>MLESKLKAPVFTATTQGDHYGEFVLEPLERGFGVTLGNPLRRILLSSIPGTAVTSVYIEDVLHEFSTIPGVKEDVVEIILNLKELVVRFLDPKMASTTLILRAEGPKEVRAGDFTPSADVEIMNPDLHIATLEEGGKLYMEVRVDRGVGYVPAERHGIKDRINAIPVDAIFSPVRRVAFQVEDTRLGQRTDLDKLTLRIWTDGSVTPLEALNQAVAILKEHLNYFANPEASLLPTPEVSKGEKRESAEEDLDLPLEELGLSTRVLHSLKEEGIESVRALLALNLKDLRNIPGIGERSLEEIRQALAKKGFTLKE[4x];>MEIKRFGRIREVIPLPPLTEIQVESYKKALQADVPPEKRENVGIQAAFKETFPIEEGDKGKGGLVLDFLEYRIGDPPFSQDECREKDLTYQAPLYARLQLIHKDTGLIKEDEVFLGHLPLMTEDGSFIINGADRVIVSQIHRSPGVYFTPDPARPGRYIASIIPLPKRGPWIDLEVEASGVVTMKVNKRKFPLVLLLRVLGYDQETLVRELSAYGDLVQGLLDEAVLAMRPEEAMVRLFTLLRPGDPPKKDKALAYLFGLLADPKRYDLGEAGRYKAEEKLGVGLSGRTLVRFEDGEFKDEVFLPTLRYLFALTAGVPGHEVDDIDHLGNRRIRTVGELMADQFRVGLARLARGVRERMVMGSPDTLTPAKLVNSRPLEAALREFFSRSQLSQFKDETNPLSSLRHKRRISALGPGGLTRERAGFDVRDVHRTHYGRICPVETPEGANIGLITSLAAYARVDALGFIRTPYRRVKNGVVTEEVVYMTASEEDRYTIAQANTPLEGDRIATDRVVARRRGEPVIVAPEEVEFMDVSPKQVFSLNTNLIPFLEHDDANRALMGSNMQTQAVPLIRAQAPVVMTGLEERVVRDSLAALYAEEDGEVVKVDGTRIAVRYEDGRLVEHPLRRYARSNQGTAFDQRPRVRVGQRVKKGDLLADGPASEEGFLALGQNVLVAIMPFDGYNFEDAIVISEELLKRDFYTSIHIERYEIEARDTKLGPERITRDIPHLSEAALRDLDEEGIVRIGAEVKPGDILVGRTSFKGEQEPSPEERLLRSIFGEKARDVKDTSLRVPPGEGGIVVGRLRLRRGDPGVELKPGVREVVRVFVAQKRKLQVGDKLANRHGNKGVVAKILPVEDMPHLPDGTPVDVILNPLGVPSRMNLGQILETHLGLAGYFLGQRYISPVFDGATEPEIKELLAEAFNLYFGKRQGEGFGVDKREKEVLARAEKLGLVSPGKSPEEQLKELFDLGKVVLYDGRTGEPFEGPIVVGQMFIMKLYHMVEDKMHARSTGPYSLITQQPLGGKAQFGGQRFGEMEVWALEAYGAAHTLQEMLTIKSDDIEGRNAAYQAIIKGEDVPEPSVPESFRVLVKELQALALDVQTLDEKDNPVDIFEGLASKR[2x];>MKKEVRKVRIALASPEKIRSWSYGEVEKPETINYRTLKPERDGLFDERIFGPIKDYECACGKYKRQRFEGKVCERCGVEVTRSIVRRYRMGHIELATPAAHIWFVKDVPSKIGTLLDLSATELEQVLYFNKYIVLDPKGAVLDGVPVEKRQLLTDEEYRELRYGKQETYPLPAGVDALVKDGEEVVKGQELAPGVVSRMDGVALYRFPRRVRVDYLRKERAALRIPLSAWVEKEAYRPGEVLAELSEPYLFRAEESGVVELKDLAEGHLIYLRQEEEVVARYFLPAGMTPLVVEGEIVEVGQPLAEGKGLLRLPRHMTAKEVEAEEEGDSVHLTLFLEWTEPKDYKVAPHMNVIVPEGAKVQAGEKIVAAIDPEEEVIAEAEGVVHLHEPASILVVKARVYPFEDDVEVTTGDRVAPGDVLADGGKVKSEIYGRVEVDLVRNVVRVVESYDIDARMGAEAIQELLKELDLEKLERELLEEMKHPSRARRAKARKRLEVVRAFLDSGNRPEWMILEAVPVLPPDLRPMVQVDGGRFATSDLNDLYRRLINRNNRLKKLLAQGAPEIIIRNEKRMLQEAVDAVIDNGRRGSPVTNPGSERPLRSLTDILSGKQGRFRQNLLGKRVDYSGRSVIVVGPQLKLHQCGLPKRMALELFKPFLLKKMEEKAFAPNVKAARRMLERQRDIKDEVWDALEEVIHGKVVLLNRAPTLHRLGIQAFQPVLVEGQSIQLHPLVCEAFNADFDGDQMAVHVPLSSFAQAEARIQMLSAHNLLSPASGEPL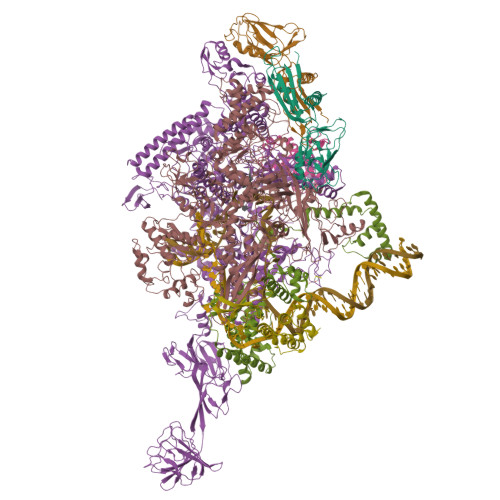AKPSRDIILGLYYITQVRKEKKGAGMAFATPEEALAAYERGEVALNAPIVVAGRETSVGRLKFVFANPDEALLAVAHGLLDLQDVVTVRYLGRRLETSPGRILFARIVGEAVGDEKVAQELIQMDVPQEKNSLKDLVYQAFLRLGMEKTARLLDALKYYGFTLSTTSGITIGIDDAVIPEEKQRYLEEADRKLRQIEQAYEMGFLTDRERYDQVIQLWTETTEKVTQAVFKNFEENYPFNPLYVMAQSGARGNPQQIRQLCGMRGLMQKPSGETFEVPVRSSFREGLTVLEYFISSHGARKGGADTALRTADSGYLTRKLVDVAHEIVVREADCGTTNYISVPLFQMDEVTRTLRLRKRSDIESGLYGRVLAREVEALGRRLEEGRYLSLEDVHFLIKAAEAGEVREVPVRSPLTCQTRYGVCQKCYGYDLSMARPVSIGEAVGVVAAESIGEPGTQLTMRTFHTGGVAVGTDITQGLPRVIELFEARRPKAKAVISEIDGVVRIEEGEDRLSVFVESEGFSKEYKLPKDARLLVKDGDYVEAGQPLTRGAIDPHQLLEAKGPEAVERYLVDEIQKVYRAQGVKLHDKHIEIVVRQMLKYVEVTDPGDSRLLEGQVLEKWDVEALNERLIAEGKVPVAWKPLLMGVTKSALSTKSWLSAASFQNTTHVLTEAAIAGKKDELIGLKENVILGRLIPAGTGSDFVRFTQVVDQRTLKAIEEARKEAVEAKEKEAPRRPVRREQPGKGL[2x];>MAEPGIDKLFGMVDSKYRLTVVVAKRAQQLLRHRFKNTVLEPEERPKMRTLEGLYDDPNAVTWAMKELLTGRLFFGENLVPEDRLQKEMERLYPTEEEA[2x];>TSDPVRQYLHEIGQVPLLTLEEEIDLARKVEEGMEAIKKLSEATGLDQELIREVVRAKILGTARIQKIPGLKEKPDPKTVEEVDGKLKSLPKELKRYLHIAREGEAARQHLIEANLRLVVSIAKKYTGRGLSFLDLIQEGNQGLIRAVEKFEYKRRFKFSTYATWWIRQAINRAIADQARTIRIPVHMVETINKLSRTARQLQQELGREPSYEEIAEAMGPGWDAKRVEETLKIAQEPVSLETPIGDEKDSFYGDFIPDENLPSPVEAAAQSLLSEELEKALSKLSEREAMVLKLRKGLIDGREHTLEEVGAYFGVTRERIRQIENKALRKLKYHESRTRKLRDFLE[2x];>[2x]MKEFRPGDKVVLPPYGVGVVAGIAQRSVSGVSRAYYQVDFPGSRSKAYVPVEAPHSVGLRKALAPEEVPVILDLLKNGRMPLPKQWAARHRKTSEILADGNPYRIAQMAGQLRAWEVERGLPDLDRQALRRAIHLLAEEVAQSLEITVQEAKRLFEEAWGEELN> MHHHHHHGSHMASAKNRRDRNSWGGFSEKTYEWSSEEEEPVKKAGPVQVLIVKDDHSFELDETALNRILLSEAVRDKEVVAVSVAGAFRKGKSFLMDFMLRYMYNQESVDWVGDYNEPLTGFSWRGGSERETTGIQIWSEIFLINKPDGKKVAVLLM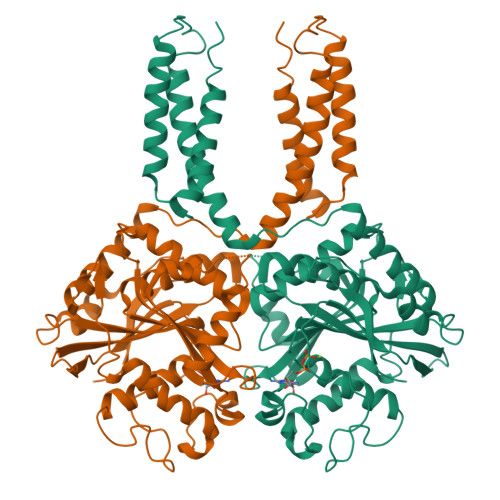DTQGTFDSQSTLRDSATVFALSTMISSIQVYNLSQNVQEDDLQHLQLFTEYGRLAMEETFLKPFQSLIFLVRDWSFPYEFSYGADGGAKFLEKRLKVSGNQHEELQNVRKHIHSCFTNISCFLLPHPGLKVATNPNFDGKLKEIDDEFIKNLKILIPWLLSPESLDIKEINGNKITCRGLVEYFKAYIKIYQGEELPHPKSMLQATAEANNLAAVATAKDTYNKKMEEICGGDKPFLAPNDLQTKHLQLKEESVKLFRGVKKMGGEEFSRRYLQQLESEIDELYIQYIKHNDSKNIFHAART>MNHKVHHHHHHMAKFFTISSSYIKYLKDFDDKVPNSEDPTYNNPKAFIGIVLEIEGHKYLAPLTSPKAWHANVKESSPAFFKLHENGVPDNQLGLINLKFMIPIIEAEVSLLDLDSMPDTPYKRMLYK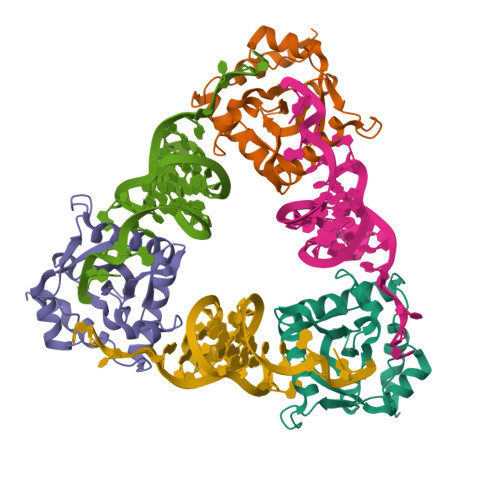QLQFIRVNEDKISEKSKLLRNLALQGRMQGTCDFAVLEEKYQHFGKKPEDMEIDDLESR[6x]> SNAMFAPQGLAQFIKVNVTLENGEPVFIYTDANGQVCQGDITVTQAGTITYLLNDQTLKGLKFVGVGFVTPFDGIIDAVTISSDGMLVQLVDLDKTPGTTKFQFVLSNTANTL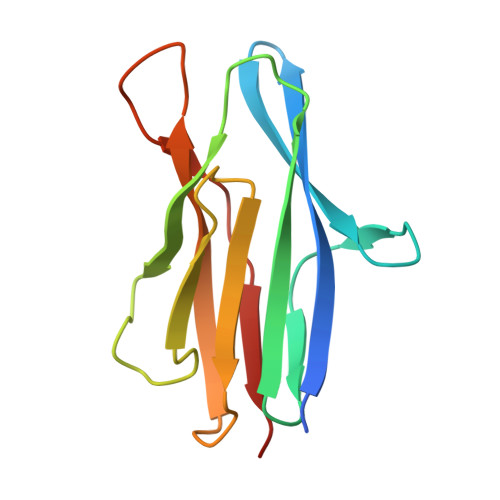LVLAPDPQIINRPQN1-(4-ethylphenyl)propan-1-one | 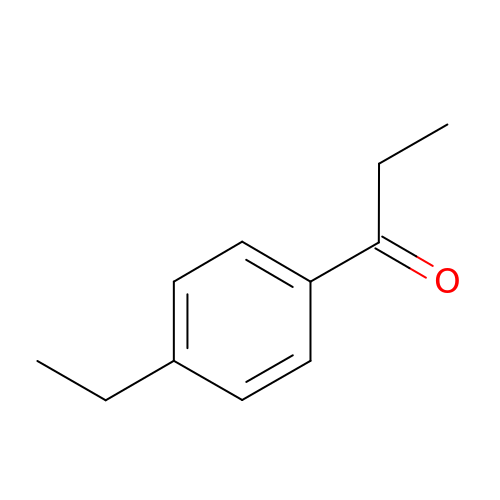C11 H14 O | VGQRIILEZYZAOE-UHFFFAOYSA-N>HHHHHHATRSPGVVISDDEPGYDLDLFCIPNHYAEDLERVFIPHGLIMDRTERLARDVMKEMGGHHIVALCVLKGGYKFFADLLDYIKALNRNSDRSIPMTVDFIRLKSYCNDQSTGDIKVIGGDDLSTLTGKNVLIVEDIIDTGKTMQTLLSLVRQYNPKMVKVASLLVKRTPRSVGYKPDFVGFEIPDKFVVGYALDY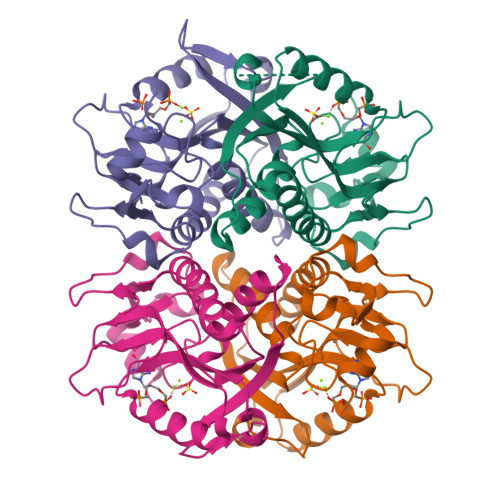NEYFRDLNHVCVISETGKAKYKA[4x]>MLKEKWWLPFLTVGVILVAVFALFYIAGPNRHNKGSTQKDGSSAVEHELTGQQLPEFEMVDQAGYQKKSA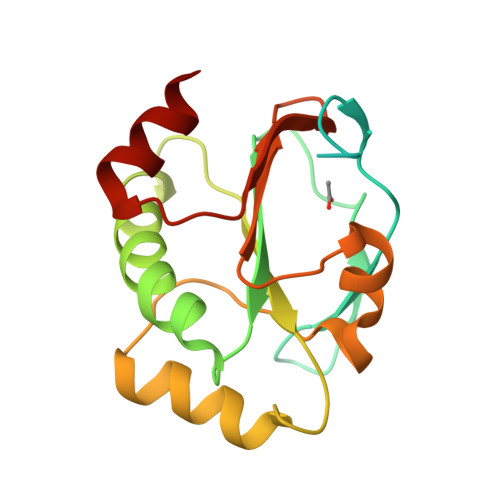EFYNKPMLVVEWASWCPDCQKQLPEIQKVYEKYKGKIHFVMLDMLDSKRETKERADQYISEKDYTFPYYYDTDERAADILHVQSIPTIYLVDKNQKVKKVMTDFHDEAALEKQLEEI[2x]>[6x]GYLGGFLLVLHSQTDQEPTCPLGMPRLWTGYSLLYLEGQEKAHNQDLGLAGSCLPVFSTLPFAYCNIHQVCHYAQRNDRS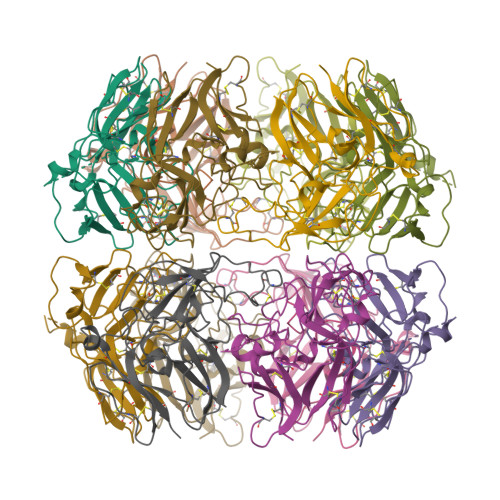YWLASAAPLPMMPLSEEAIRPYVSRCAVCEAPAQAVAVHSQDQSIPPCPQTWRSLWIGYSFLMHTGAGDQGGGQALMSPGSCLEDFRAAPFLECQGRQGTCHFFANKYSFWLTTVKADLQFSSAPAPDTLKESQAQRQKISRCQVCVKYS> MAAIQGIEGVISQLQ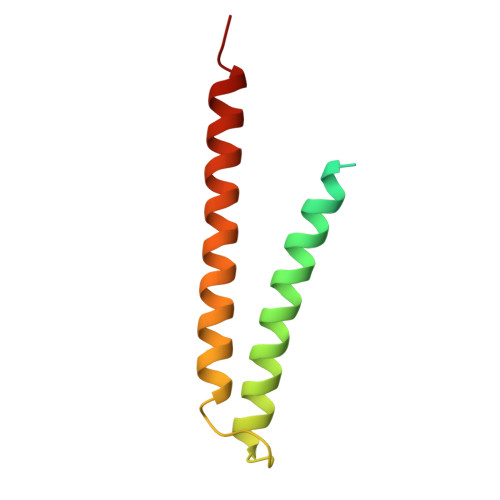ATAMAARGQDTHSQSTVSFAGQLHAALDRISDRQAAARVQAEKFTLGEPGIALNDVMADMQKASVSMQMGIQVRNKLVAAYQEVMSMQV>MDAEGLALLLPPVTLAALVDSWLREDCPGLNYAALVSGAGPSQAALWAK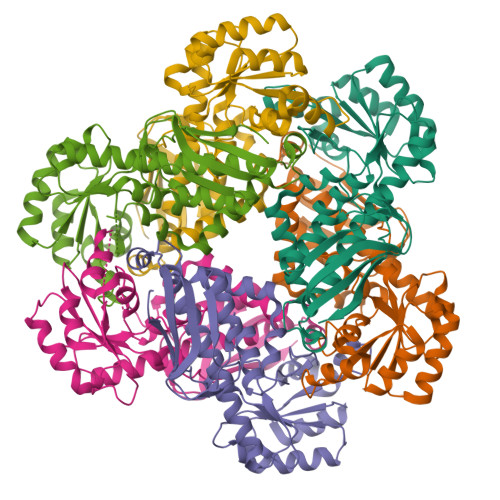SPGVLAGQPFFDAIFTQLNCQVSWFLPEGSKLVPVARVAEVRGPAHCLLLGERVALNTLARCSGIASAAAAAVEAARGAGWTGHVAGTRKTTPGFRLVEKYGLLVGGAASHRYDLGGLVMVKDNHVVAAGGVEKAVRAARQAADFTLKVEVECSSLQEAVQAAEAGADLVLLDNFKPEELHPTATVLKAQFPSVAVEASGGITLDNLPQFCGPHIDVISMGMLTQAAPALDFSLKLFAKEVAPVPKIHLEHHHHHH[6x]> GSSRTELLNVCMNAKHHKEKPGPEDKLHEQCRPWRKNACCSTNTSQEAHKDVSYLYRFNWNHCGEMAPACKRHFIQDTCLYECSPNLGPWIQQVDQSWRKERVLNVPLCKEDCEQWWEDCRTSYTCKSNWHKGWNWTSGFNKC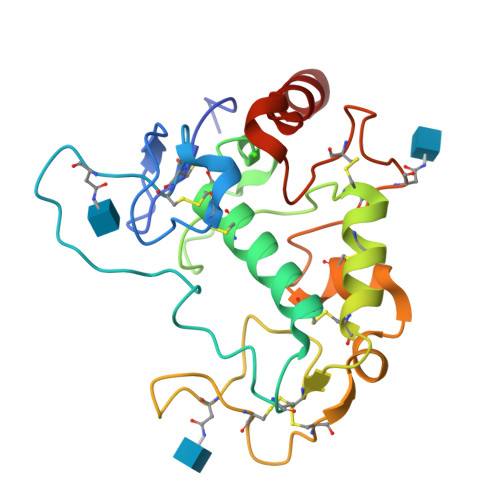AVGAACQPFHFYFPTPTVLCNEIWTHSYKVSNYSRGSGRCIQMWFDPAQGNPNEEVARFYAAAMS> GAENESTPIQQLLEHFLRQLQRKDP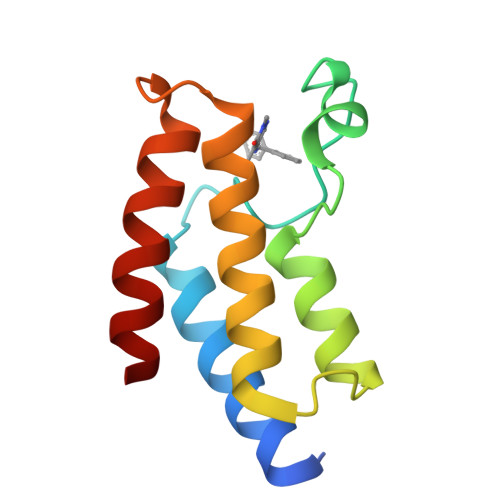HGFFAFPVTDAIAPGYSMIIKHPMDFGTMKDKIVANEYKSVTEFKADFKLMCDNAMTYNRPDTVYYKLAKKILHAGFKMMS> MATLTAKNLAKAYKGRRVVEDVSLTVNSGEIVGLLGPNGAGKTTTFYMVVGIVPRDAGNIIIDDEDISLLPLHARARRGIGYLPQEASIFRRLSVFDNLMAVLQIRDDLTSEQRQDRANELMEEFHIEHLRDSLGQ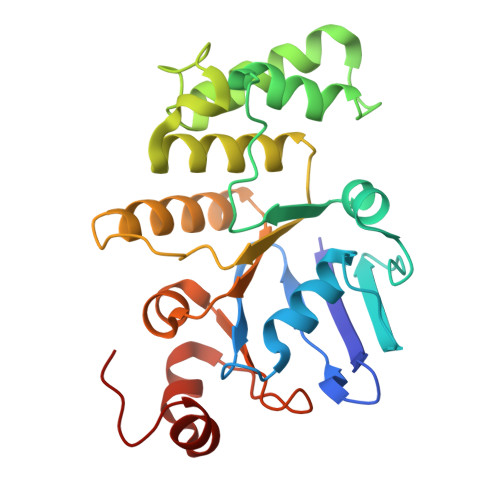ALSGGERRRVEIARALAANPKFILLDEPFAGVDPISVIDIKRIIEHLRDSGLGVLITDHNVRETLAVCERAYIVSQGNLIAHGTPQQILEDDHVKRVYLGEDFRL> MHHHHHHHHAGPRGVRRILPFLGPAVIASIAYMDPGNFATNIEGGARYGYSLLWVILAANLMAMVIQNLSANLGIASGRNLPELIRERWPRPLVWFYWIQAELVAMATDLAEFLGAALAIQLLTGLPMFWGAVVTGVVTFWLLNLQKRGTRPLELAVGAFVLMIGVAYLVQVVLARPDLAAVGAGFVPRLQGPGSAYLAVGIIGATVMPHVIYLHSALTQGRIQTDTTEEKRRLVRLNRVDVIAAMGLAGLINMSMLAVAAATFHGKNVENAGALTTAYQTLTPLLGPAASVLFAVALLASGLSSSAVGTMAGDVIMQGFMGFHIPLWLRRLITMLPAFIVILLGMDPSSVLILSQVILCFGVPFALVPLLLFTARRDVMGALVTRRSFTVIGWVIAVIIIALNGYLLWELLGG

Transporters of the Nramp (Natural resistance-associated macrophage protein) family import divalent transition metal ions into cells of most organisms. In addition to the physiological substrates Fe2+ and Mn2+, Nramps can also transport toxic metals like Cd2+ and Hg2+ but exclude the abundant alkaline earth metals like Mg2+ and Ca2+. Recent bacterial Nramp structures reveal a LeuT fold, three stable conformations (outward-open, occluded, and inward-open), and identify the metal-binding site residues, including conserved aspartate, asparagine, and methionine residues. We present high-resolution structures of DraNramp in three conformations in both Mn2+-bound and metal-free states, providing the first molecular map of the entire Mn2+ transport cycle.

Two new structures of DraNramp point-mutants reveal the coordination of Mn2+ in the inward-open state: M230A•Mn2+ and D296A•Mn2+ (Cα RMSD of 0.42 Å). The Mn2+ is in the same location of the orthosteric site as in the occluded state, as confirmed by anomalous diffraction for D296A•Mn2+. (A) Cartoon representation of the inward-open structure of D296A•Mn2+, which is nearly identical to the M230A•Mn2+ inward-open structure (Cα RMSD of 0.38 Å). (B) Coordination sphere of the orthosteric Mn2+ ion in the D296A structure is nearly the same as in M230A Mn2+-bound structure except for the sulfur of M230 replacing a water seen in M230A. We do not observe a bound water to complete the coordination sphere of D296A, likely because the resolution of the structure is lower (2.52 Å for M230A•Mn2+ vs. 3.12 Å for D296A•Mn2+), otherwise the structures are analogous. The peak from the anomalous difference Fourier map (magenta mesh; 4.5σ) calculated from a D296A•Mn2+ crystal confirms a bound Mn2+ in this inward-open state. The D296A and D369A variants each bind one Mn2+ with Kd=370±30 µM and 420±30 µM respectively, which is closest to Kd1 of WT. The occluded and inward-open states may be energetically similar as relatively small perturbations yielded inward-open structures (M230A•Mn2+ and D296A•Mn2+).> MGHHHHHHSAKQTGYLTIGGQRYQAEINDLENLGEMGSGTCGQVWKMRFRKTGHVIAVKQMRRSGNKEENKRILMDLDVVLKSHDCPYIVQCFGTFITNTDVFIAMELMGTCAEKLKKRMQGPIPERILGKMTVAIVKALYYLKEKHGVIHRDVKPSNILLDERGQIKLCDFGISGRLVDSKAKTRSAGCAAYMAPERIDPPDPTKPDYDIRADVWS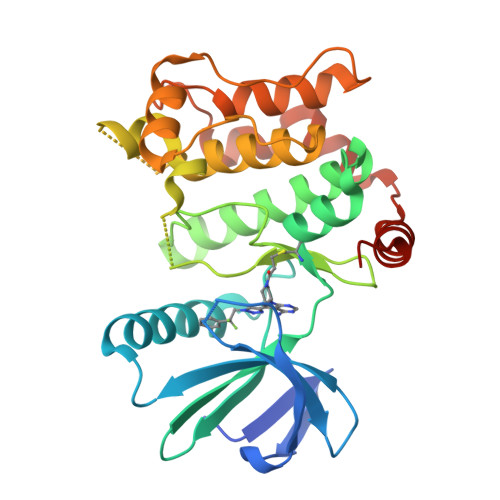LGISLVELATGQFPYKNCKTDFEVLTKVLQEEPPLLPGHMGFSGDFQSFVKDCLTKDHRKRPKYNKLLEHSFIKRYETLEVDVASWFKDVMAKTRSPRTSG>MERAIQGNDTREQANGERWDGGSGGITSPFKLPDESPSWTEWRLYNDETNSNQDNPLGFKESWGFGKVVFKRYLRYDRTEASLHRVLGSWTGDSVNYAASRFLGANQVGCTYSIRFRGVSVTISGGSRTLQHLCEMAIRSKQELLQLTPVEVESNVSRGCP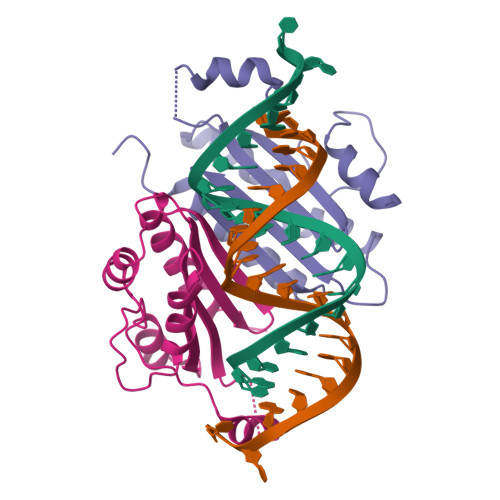EGIETFKKESE[2x]> MGGSSHHHHHHSSGLVPRGSHMKLITASSSKEYLPDLLLFWQNYEYWITNIGLYKTKQRDLTRTPANLDTDTEECMFWMNYLQKDQSFQLMNFAMENL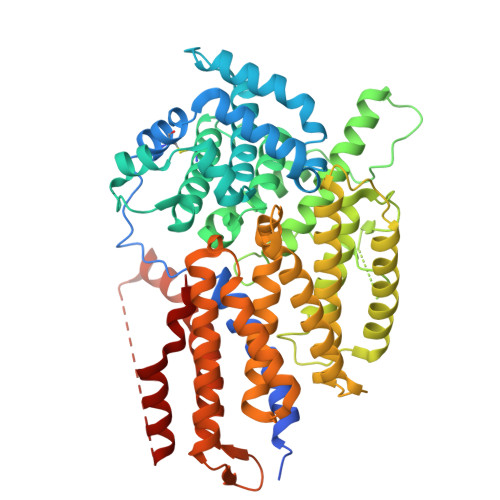GALYFGSIGDISELYLRVEQYWDRRADKNHSVDGKYWDALIWSVFTMCIYYMPVEKLAEIFSVYPLHEYLGSNKRLNWEDGMQLVMCQNFARCSLFQLKQCDFMAHPDIRLVQAYLILATTTFPYDEPLLANSLLTQCIHTFKNFHVDDFRPLLNDDPVESIAKVTLGRIFYRLCGCDYLQSGPRKPIALHTEVSSLLQHAAYLQDLPNVDVYREENSTEVLYWKIISLDRDLDQYLNKSSKPPLKTLDAIRRELDIFQYKVDSLEEDFRSNNSRFQKFIALFQISTVSWKLFKMYLIYYDTADSLLKVIHYSKVIISLIVNNFHAKSEFFNRHPMVMQTITRVVSFISFYQIFVESAAVKQLLVDLTELTANLPTIFGSKLDKLVYLTERLSKLKLLWDKVQLLDSGDSFYHPVFKILQNDIKIIELKNDEMFSLIKGLGSLVPLNKLRQESLLEEEDENNTEPSDFRTIVEEFQSEYNISDILS> NDDKLYRADSRP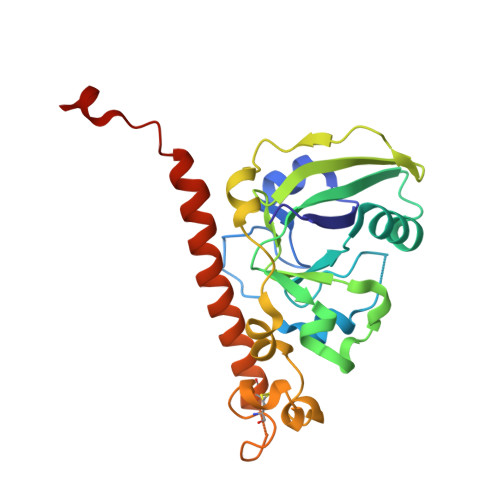PDEIKQSGGLMPRGQSEYFDRGTQMNINLYDHARGTQTGFVRHDDGYVSTSISLRSAHLVGQTILSGHSTYYIYVIATAPNMFNVNDVLGAYSPHPDEQEVSALGGIPYSQIYGWYRVHFGVLDEQLHRNRGYRDRYYSNLDIAPAADGYGLAGFPPEHRAWREEPWIHHAPPGCGNAPRSSMSNTCDEKTQSLGVKFLDEYQSKVKRQIFSGYQSDIDTHNRIKDEL4-(6-ethoxypyrazolo[1,5-b]pyridazin-3-yl)-~{N}-[3-methoxy-5-(trifluoromethyl)phenyl]pyrimidin-2-amine 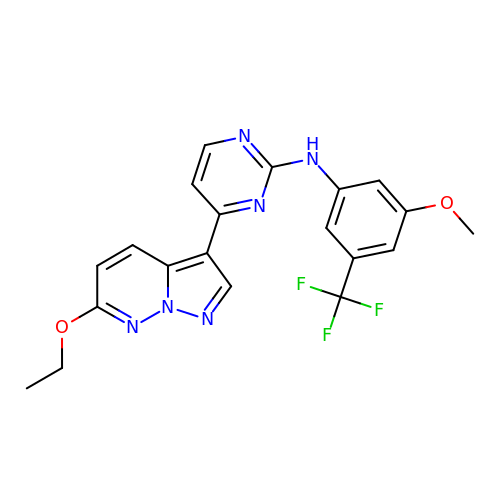| C20 H17 F3 N6 O2 | FXUBIYKZSFWJQZ-UHFFFAOYSA-N6-(2-{3-(aminomethyl)-5-[2-(1H-pyrrolo[2,3-b]pyridin-6-yl)ethyl]phenyl}ethyl)-4-methylpyridin-2-amine 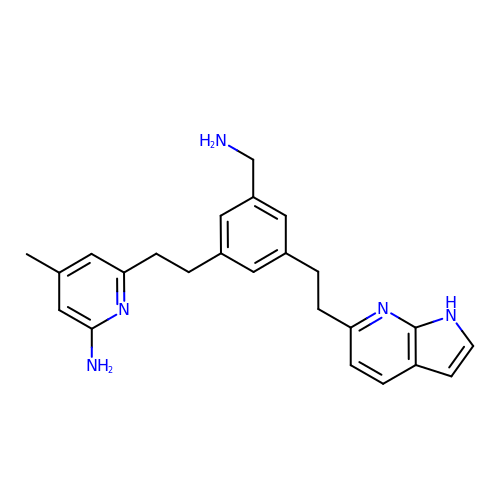| C24 H27 N5 | WRRLIUHCTMZNNL-UHFFFAOYSA-N>[4x]MKRLEGKVAIVTSSTRGIGRASAEALAKEGALVYLAARSEELANEVIADIKKQGGVAKFVYFNAREEETYTSMVEKVAEAEGRIDILVNNYGGTN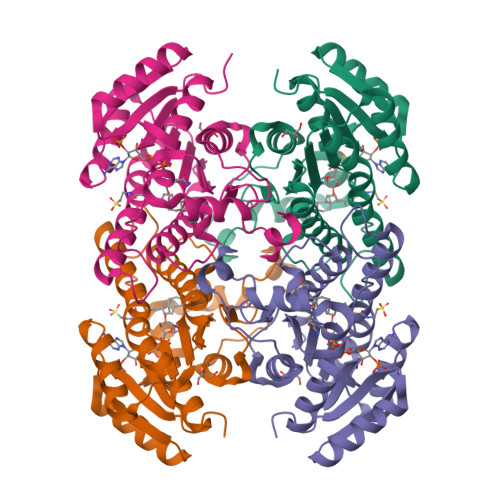VNLDKNLTAGDTDEFFRILKDNVQSVYLPAKAAIPHMEKVGGGSIVNISTIGSVVPDISRIAYCVSKSAINSLTQNIALQYARKNIRCNAVLPGLIGTRAALENMTDEFRDSFLGHVPLNRVGRPEDIANAVLYYASDDSGYVTGMIHEVAGGFALGTPQYSEYCPR> MENYLDLFSHKNMKLKERVLIPVKQYPKFNFVGKILGPQGNTIKRLQEETGAKISVLGKGSM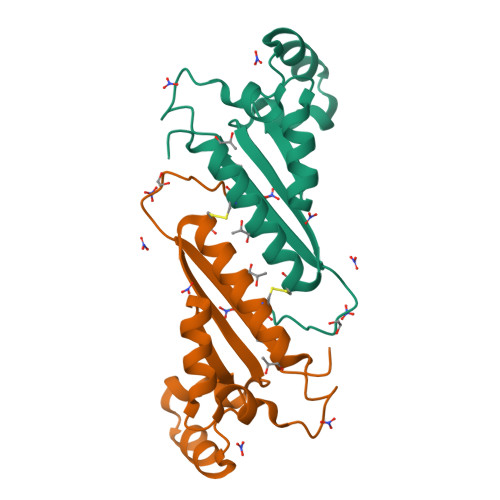RDKAKEEELRKGGDPKYAHLNMDLHVFIEVFGPPCEAYALMAHAMCEVKKFLVPDM>[2x]RVTMNEFEYLKLLGKGTFGKVILVKEKATGRYYAMKILKKEVIVAKDEVAHTLTENRVLQNSRHPFLTALKYSFQTHDRLCFVMEYANGGELFFHLSRERVFSEDRARFYGAEIVSALDYLHSEKNVVYRDLKLENLMLDKDGHIKITDFGLCKEGIKDGATMKTFCGTPEYLAPEVLEDNDYGRAVDWWGLGVVMYEMMCGRL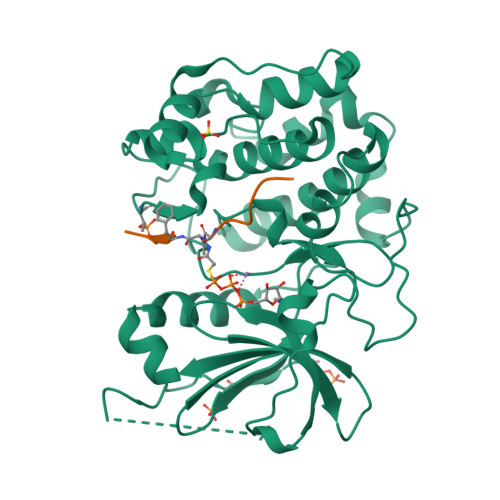PFYNQDHEKLFELILMEEIRFPRTLGPEAKSLLSGLLKKDPKQRLGGGSEDAKEIMQHRFFAGIVWQHVYEKKLSPPFKPQVTSETDTRYFDEEFTAQMITITPPDQDDSMECVDSERRPHFPQFSYSASGTA;>GRPRTTXFAE[2x]Ribonucleotide reductases (RNRs) catalyze the conversion of ribonucleotides to deoxyribonucleotides, a conserved reaction that is fundamental to DNA-based life. Nearly all aerobic organisms use class I RNRs, which consist of two subunits: α, which contains the catalytic site, and β, which houses a subclass-dependent metal center. Contrary to all other class Ib RNRs studied to-date, the sole RNR of Bacillus subtilis displays class Ia-like activity regulation. We find that B. subtilis RNR has arrived at a remarkably similar solution to the ATP-cone through the evolution of two unique allosteric sites that modulate catalytic activity by inducing contrasting quaternary interactions that either enable or prevent the full range of motions needed for RNR activity.

Because enzyme activity requires both α and β subunits, cryo-EM was repeated with mixtures of holo-NrdE and NrdF (abbreviated as “NrdEF”) under inhibiting conditions. The resultant cryo-EM map revealed a NrdEF filament consisting of a single-helical NrdE strand (gray surface) with EM density corresponding to NrdF observed at higher contour levels filling the helical interior (green). The resolution of the reconstruction varied across the map, as high-resolution features were distinguishable in NrdE but not in NrdF. Additional density was observed in a hydrophobic cleft of NrdE (green) that was previously shown to bind the β C-terminus in other class I RNRs. Density for the NrdF core is significantly weaker than the remainder of the NrdEF map, but density for the NrdF C-terminus is observed at similar thresholds as NrdE. This discrepancy suggests that the NrdF core is flexibly linked to NrdE by NrdF C-termini, resulting in high occupancy but significant variability in orientation. Attempts to refine the map from biased initial models with little gap between NrdE and NrdF invariably converged to have a pronounced gap of roughly 15–20  Å between the subunits (see the section “Methods”). Thus, instead of forming a buried interface with NrdE, the NrdF core density is on average placed far from the catalytic sites. For both filaments, excess density at the S-site was modeled as dATP.

>[2x]MSQNQVPKWIQLNNEIMIQKDGKFQFDKDKEAVHSYFVDYINQNTVFFHNLKEKLDYLVENQYYEEEFLSLYSFEDIKEVFKTAYAKKFRFPSFMSAFKFYNDYALKTNDKKKILERYEDRISIVALFFANGDTEKAKEYVNLMINQEYQPSTPTFLNAGRKRRGELVSCFLLEVNDSLNDISRAIDISMQLSKLGGGVSLNLSKLRAKGEAIKDVENATKGVVGVMKLLDNAFRYADQMGQRQGSGAAYLNIFHRDINDFLDTKKISADEDVRVKTLSIGVVIPDKFVELAREDKAAYVFYPHTIYKEYGQHMDEMDMNEMYDKFVDNPRVKKEKINPRKLLEKLAMLRSESGYPYIMFQDNVNKVHANNHISKVKFSNLCSEVLQASQVSSYTDYDEEDEIGLDISCNLGSLNILNVMEHKSIEKTVKLATDSLTHVSETTDIRNAPAVRRANKAMKSIGLGAMNLHGYLAQNGIAYESPEARDFANTFFMMVNFYSIQRSAEIAKEKGETFDQYEGSTYATGEYFDKYVSTDFSPKYEKIANLFEGMHIPTTEDWKKLKAFVAEHGMYHSYRLCIAPTGSISYVQSSTASVMPIMERIEERTYGNSKTYYPMPGLASNNWFFYKEAYDMDMFKVVDMIATIQQHIDQGISFTLFLKDTMTTRDLNRIDLYAHHRGIKTIYYARTKDTGQDSCLSCVV> SPIQVIENDRASRGGQVYATNTRGQIPPLVTTDCMIQDQGNASPRFIRCTTYCFPCTSDMAKQAQIPLAAVIKPFATIPSNESPLYLVNHGESGPVRCNRCKAYMCPFMQFIEGGRRYQCGFCNCVNDVPPFYFQHLDHIGRRLDHYEKPELSLGSYEYVATLDYCRKSKPPNPPAFIFMIDVSYSNIKNGLVKLICEELKTMLEKIPKEEQEETSAIRVGFITYNKVLHFFNVKSNLAQPQMMVVTDVGEVFVPLLDGFLVNYQESQSVIHNLLDQIPDMFADSNENETVFAPVIQAGMEALKAADCPGKLFIFHSSLPTAEAPGKLKNRDDKKLVNTDKEKILFQPQTNVYDSLAKDCVAHGCSVTLFLFPSQYVDVASLGLVPQLTGGTLYKYNNFQMHLDRQQFLNDLRNDIEKKIGFDAIMRVRTSTGFRATDFFGGILMNNTTDVEMAAIDCDKAVTVEFKH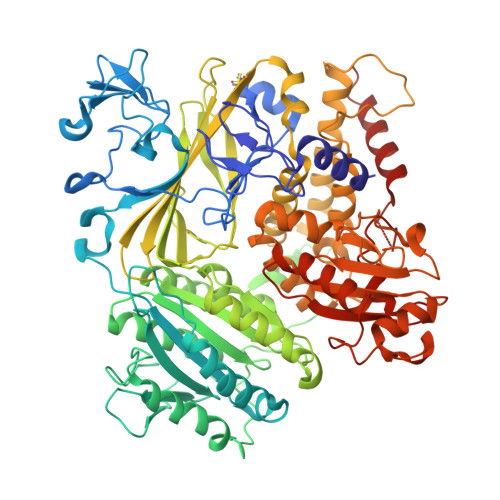DDKLSEDSGALIQCAVLYTTISGQRRLRIHNLGLNCSSQLADLYKSCETDALINFFAKSAFKAVLHQPLKVIREILVNQTAHMLACYRKNCASPSAASQLILPDSMKVLPVYMNCLLKNCVLLSRPEISTDERAYQRQLVMTMGVADSQLFFYPQLLPIHTLDVKSTMLPAAVRCSESRLSEEGIFLLANGLHMFLWLGVSSPPELIQGIFNVPSFAHINTDMTLLPEVGNPYSQQLRMIMGIIQQKRPYSMKLTIVKQREQPEMVFRQFLVEDKGLYGGSSYVDFLCCVHKEICQLLN> SNAMALPRITDYPLPTAAELPQARGPWRPQRDRVALLVHDMQRYFLAAFDAGNAPLRPAVDNIARLLAHCRARGIPVFYTAQHGDQDRRDRGLQADLWGPGMRRSADHEPIIDALAPQPGEHVLVKHRYSAFQRSNLETLMRVRGRDQLLVTGVYAHIGCTATVVEAFQRDIEAFIAADAVADFSRADHDQALHWIARTSGVPMT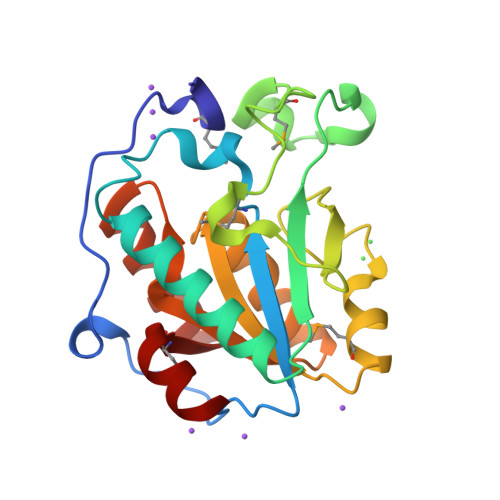TDQLLEVL> MPSLPTLQPLDLYRRTLACLV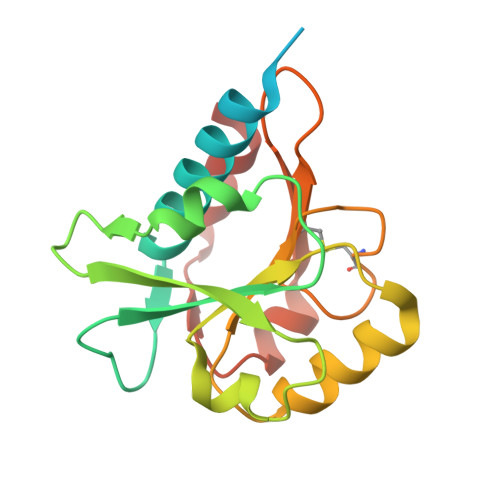LAVSCLGGGGLWADDARTSIEQRSNAVSQVLLGIFSYVRWPKEPAVLQLCVVGPTEYADGLLRGMVQANGRRVHAERRAVDNPDLGTLCNVIYLGVVDERERQQVFRSLAGHPVLSISERGTECSVGSMFCLNVGGPRITFEANLDSIARSGVRVHPSVLKLARRQATP>[2x]MGGYVNIKTFTHPAGEGKEVKGMEVSVPFEIYSNEHRIADAHYQT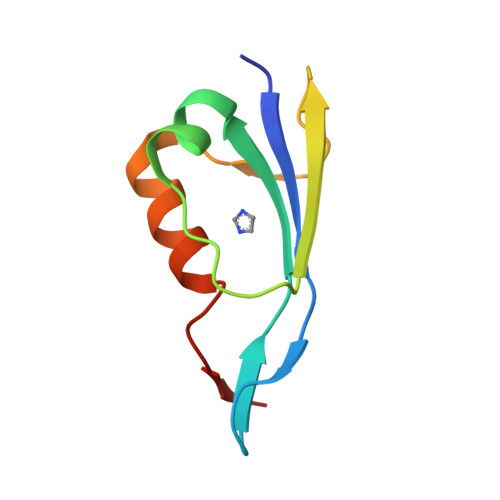FPSEKAAYTTVVTDAADWRTKNAAMFTPTPVSG>DVGCSVDFSKKETRCGTGVFIYNDVEAWRDRYKYHPDSPRRLAAAVKQAWEEGICGISSVSRMENIMWKSVEGELNAILEENGVQLTVVVGSVKNPMWRGPQRLPVPVNELPHGWKAWGKSYFVRAAKTNNSFVVDGDTLKECPLEHRAWNSFLVEDHGFGVFHTSVWLKVREDYSLECDPAVIGTAVKGREAAHSDLGYWIESEKNDTWRLKRAHLIEMKTCEWPKSHTLWTDGVEESDLIIPKSLAGPLSHHNTREGYRTQVKGPWHSEELEIRFEECPGTKVYVEETCGTRGPSLRSTTASGRVIEEWCCRECTMPPLSFRAKDGCWYGMEIRPRKEPESNLVRSMVTAGTKHHHHHH[4x]

The non-structural protein 1 (NS1) is secreted from the infected cell and is thought to be associated with disease severity besides its proven usefulness for differential diagnoses. NS1 can be found intracellularly, where it is essential for virus replication, docked on lipid rafts of the cell surface membrane, and abundantly secreted into the bloodstream of infected individuals during the febrile phase. NS1 is comprised of three distinct domains, an N-terminal hydrophobic β-roll dimerization domain (residues 1–29) formed by the intertwining of two protomers, an α/β-wing domain (residues 38–151) that extends out from the central β-ladder domain (residues 181–352) giving the dimer a distinct crossed shape. Here, we present high-resolution cryoEM structures of ZIKV recombinant secreted NS1 (rsNS1) and its complexes with three human monoclonal antibodies (AA12, EB9, GB5), as well as evidence for ZIKV infection-derived secreted NS1 (isNS1) binding to High Density Lipoprotein (HDL).

We expressed and purified full-length recombinant ZIKV NS1 (Uganda strain MR766; Zv sNS1MR766wt) with a carboxy (C)-terminus poly-histidine (HIS)-tag from the supernatant of transfected Expi293 cells. To achieve a higher resolution cryoEM structure of ZIKV rsNS1, we obtained a suitable dataset for single-particle analysis by increasing the sample concentration on graphene grids. We similarly observed asymmetric tetramers and achieved an improved cryoEM map of 2.9 Å, although the distal ends of the β-ladder and wing domains are poorly resolved and there is significant smearing in one of the dimers. While focus refinements on the individual dimers did not improve the overall accuracy of the map, they showed obvious movement between them. We proceeded using the overall tetramer map to model all the residues, including uncertain regions such as the flexible loop at the wing tip, for completeness and interpretation of the protein movement. The range of motion hinges around the β-roll interface with movements up to 15.02° rotation. The dimer-dimer interface consists of the β-rolls oriented almost perpendicularly to each other with potential interactions between Phe163 in the greasy finger of the wing domain and Asp274 of the β-ladder within 3.5 Å at the opposite protomer or other residues resulting in the assymetric tetramers. We observed tetramers of ZIKV rsNS1 (dimer of dimer), similar to the “loose” tetramers reported at 8.3 Å by Shu et al.. We first superimposed our ZIKV NS1 tetramer map with the “loose” tetrameric rsNS1 of DENV2 PVP94/07 clinical strain (EMDB-32842)24 and observed that they largely overlapped. Overall, our tetrameric ZIKV rsNS1 is highly similar to the other reported structures (RMSD:1.93), although our model showed a different angle within the trajectory of the dimer scaffold.> MVHYRTIDSPIGPLTLAGHGSVLTNLRMLEQTYEPSLTHWTPDPGAFSGAVDQLNAYFAGELTEFDVELDLRGTDFQQRVWKALLTIPYGETRSYGEIADQIGAPGAARAVGLANGHNPIAIIVPCHRVIGASGKL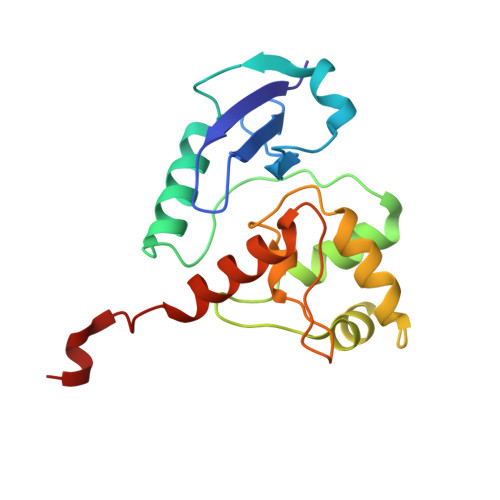TGYGGGINRKRALLELEKSRAPADLTLFD1-[(3~{R},4~{R})-4-(cyanomethyl)-3-fluoranyl-1-[(4-phenylphenyl)methyl]piperidin-4-yl]-3-(cyclopropylcarbonylamino)pyrazole-4-carboxamide | C28 H29 F N6 O2 | 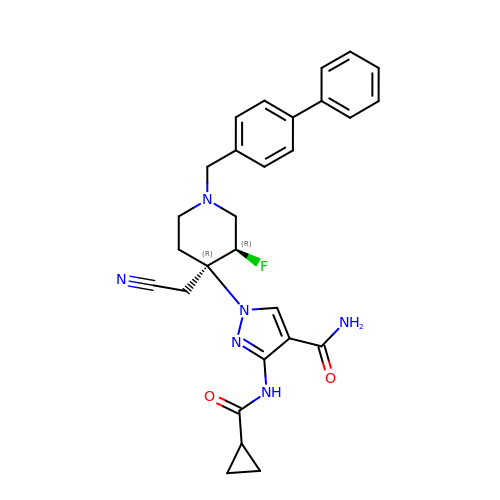MQWQEBHHQHORKK-YWEHKCAJSA-N> ELTPDQQTLLHFIMDSYNKQRMPQEITNKILKEEFSAEENFLILTEMATNHVQVLVEFTKKLPGFQTLDHEDQIALLKGSAVEAMFLRSAE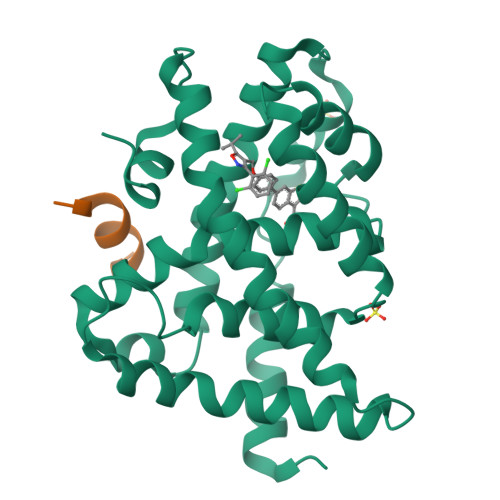IFNKKLPSGHSDLLEERIRNSGISDEYITPMFSFYKSIGELKMTQEEYALLTAIVILSPDRQYIKDREAVEKLQEPLLDVLQKLCKIHQPENPQHFACLLGRLTELRTFNHHHAEMLMSWRVNDHKFTPLLCEIWDVQ;> DHQLLRYLLDK> TVTKVSLPEGSFKRVKPQYDEIHIPAPSKPVIDYELKEITSLPDWCQEAFPSSETTSLNPIQSKVFHAAFEGDSNMLICAPTGSGKTNIALLTVLKALSHHYNPKTKKLNLSAFKIVYIAPLKALVQEQVREFQRRLAFLGIKVAELTGDSRLSRKQIDETQVLVSTPEKWDITTRNSNNLAIVELVRLLIIDEIHLLHDDRGPVLESIVARTFWASKYGQEYPRIIGLSATLPNYEDVGRFLRVPKEGLFYFDSSFRPCPLSQQFCGIKERNSLKKLKAMNDACYEKVLESINEGNQIIVFVHSRKETSRTATWLKNKFAEENITHKLTKNDAGSKQILKTEAANVLDPSLRKLIESGIGTHHAGLTRSDRSLSEDLFADGLLQVLVCTATLAWGVNLPAHTVIIKGTDVYSPEKGSWEQLSPQDVLQMLGRAGRPRYDTFGEGIIITDQSNVQYYLSVLNQQLPIESQFVSKLVDNLNAEVVAGNIKCRNDAVNWLAYTYLYVRMLASPMLYKVPDISSDGQLKKFRESLVHSALCILKEQELVLYDAENDVIEATDLGNIASSFYINHASMDVYNRELDEHTTQIDLFRIFSMSEEFKYVSVRYEEKRELKQLLEKAPIPIREDIDDPLAKVNVLLQSYFSQLKFEGFALNSDIVFIHQNAGRLLRAMFEICLKRGWGHPTRMLLNLCKSATTKMWPTNCPLRQFKTCPVEVIKRLEASTVPWGDYLQLETPAEVGRAIRSEKYGKQVYDLLKRFPKMSVTCNAQPITRSVMRFNIEIIADWIWDMNVHGSLEPFLLMLEDTDGDSILYYDVLFITPDIVGHEFTLSFTYELKQHNQNNLPPNFFLTLISENWWHSEFEIPVSFNGFKLPKKFPPPTPLLENISISTSELGNDDFSEVFEFKTFNKIQSQVFESLYNSNDSVFVGSGKGTGKTAMAELALLNHWRQNKGRAVYINPSGEKIDFLLSDWNKRFSHLAGGKIINKLGNDPSLNLKLLAKSHVLLATPVQFELLSRRWRQRKNIQSLELMIYDDAHEISQGVYGAVYETLISRMIFIATQLEKKIRFVCLSNCLANARDFGEWAGMTKSNIYNFSPSERIEPLEINIQSFKDVEHISFNFSMLQMAFEASAAAAGNRNSSSVFLPSRKDCMEVASAFMKFSKAIEWDMLNVEEEQIVPYIEKLTDGHLRAPLKHGVGILYKGMASNDERIVKRLYEYGAVSVLLISKDCSAFACKTDEVIILGTNLYDGAEHKYMPYTINELLEMVGLASGNDSMAGKVLILTSHNMKAYYKKFLIEPLPTESYLQYIIHDTLNNEIANSIIQSKQDCVDWFTYSYFYRRIHVNPSYYGVRDTSPHGISVFLSNLVETCLNDLVESSFIEIDDTEAEVTAEVNGGDDEATEIISTLSNGLIASHYGVSFFTIQSFVSSLSNTSTLKNMLYVLSTAVEFESVPLRKGDRALLVKLSKRLPLRFPEHTSSGSVSFKVFLLLQAYFSRLELPVDFQNDLKDILEKVVPLINVVVDILSANGYL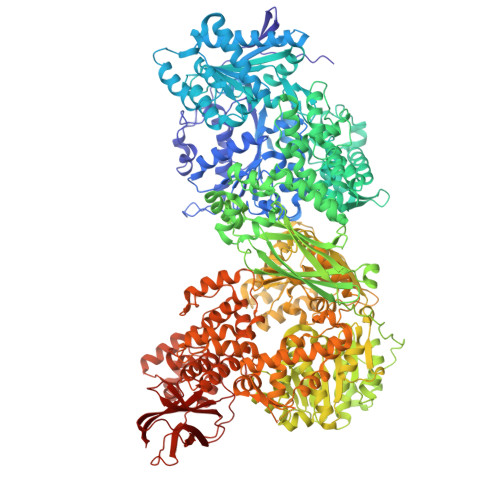NATTAMDLAQMLIQGVWDVDNPLRQIPHFNNKILEKCKEINVETVYDIMALEDEERDEILTLTDSQLAQVAAFVNNYPNVELTYSLNNSDSLISGVKQKITIQLTRDVEPENLQVTSEKYPFDKLESWWLVLGEVSKKELYAIKKVTLNKETQQYELEFDTPTSGKHNLTIWCVCDSYLDADKELSFEINVK>[8x]MKKTKIVCTIGPKTESEEMLAKMLDAGMNVMRLNFSHGDYAEHGQRIQNLRNVMSKTGKTAAILLDTKGPEIRTMKLEGGNDVSLKAGQTFTFTTDKSVIGNSEMVAVTYEG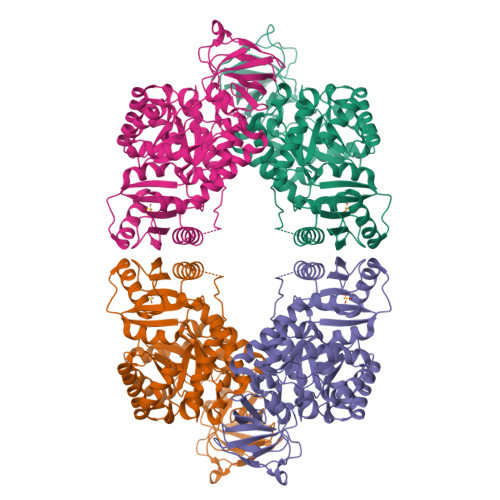FTTDLSVGNTVLVDDGLIGMEVTAIEGNKVICKVLNNGDLGENKGVNLPGVSIALPALAEKDKQDLIFGCEQGVDFVAASFIRKRSDVIEIREHLKAHGGENIHIISKIENQEGLNNFDEILEASDGIMVARGDLGVEIPVEEVIFAQKMMIEKCIRARKVVITATQMLDSMIKNPRPTRAEAGDVANSILDGTDAVMLSGESAKGKYPLEAVSIMATICERTDRVMNSRLEFNNDNRKLRITEAVCRGAVETAEKLDAPLIVVATQGGKSARAVRKYFPDATILALTTNEKTAHQLVLSKGVVPQLVKEITSTDDFYRLGKELALQSGLAHKGDVVVMVSGALVPSGTTNTASVHVL>[2x]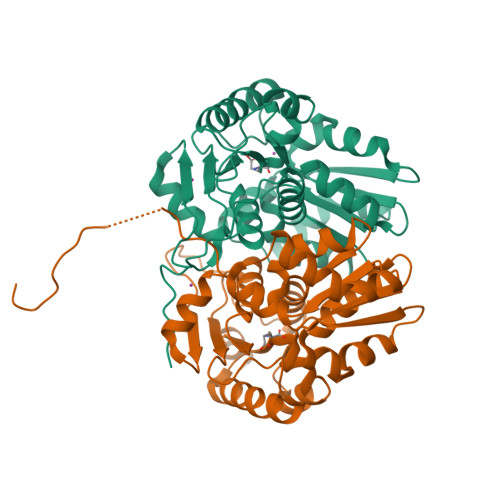SHMSDRLAPIGIFDSGVGGLTVARAIIDQLPDEDIVYVGDTGNGPYGPLTIPQIRAHSLAIGDDLVSRGVKALVIACNTASSACLRDARERYSPVPVVEVILPAVRRAVAATRNGRIGVIGTQATIASGAYQDAFAAARDTEVFTVACPRFVDFVERGVTSGRQVLGLAEGYLEPLQLAEVDTLVLGCTHYPMLSGLIQLAMGDNVTLVSSAEETAKDLLRVLTELDLLRPHPDDPSVTAVRRFEATGDPEAFTALAARFLGPTLDGVRPVRRHAGAGR> MAKRKARAVSAPVTLSEISEIPNEVTNAEDSVNELETTPTEIVSTESSENENTTADSENTAATDSTTDEESEDTSSTEANGDGESEEPDLSENQEDPKEPIETPEEPVEDDDGSGDPDGGTSEEKPTEGDPEDPEEPTEPTDPEEPTDPVDPVEPPPEEPKAFQLNLATVKSQFGDLPTYWAIELIKRYFSAPPAIYIPDVVDNPDFKIMVQQVKFFGNGLRPIY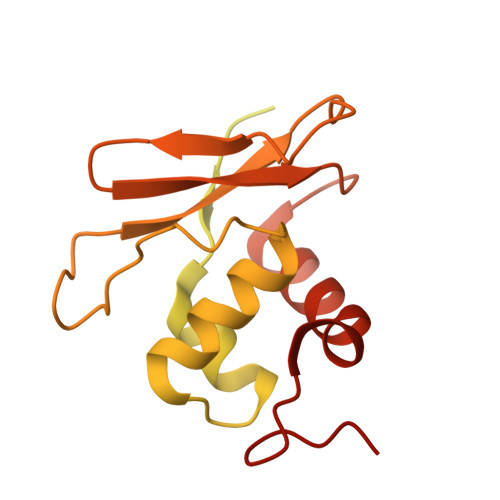NSKNMITFTTMLEGASEATILEDMKKQQPALLSLLPWYDPNAEIDK[1-[4-chloranyl-3-(trifluoromethyl)phenyl]-1,2,3-triazol-4-yl]methanol | C10 H7 Cl F3 N3 O 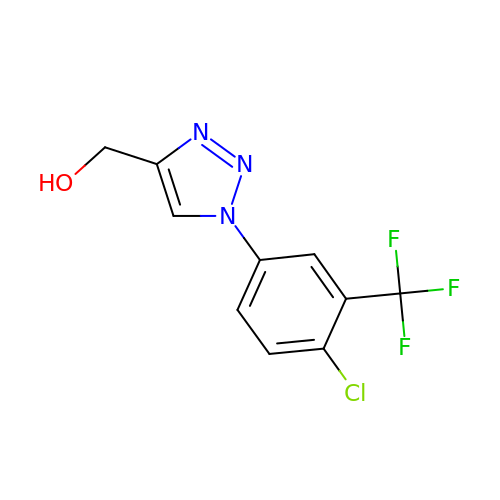| MTSIIXPDVHCKBB-UHFFFAOYSA-N> RDFNNLTKGLCTINSWHIYGKDNAVRIGED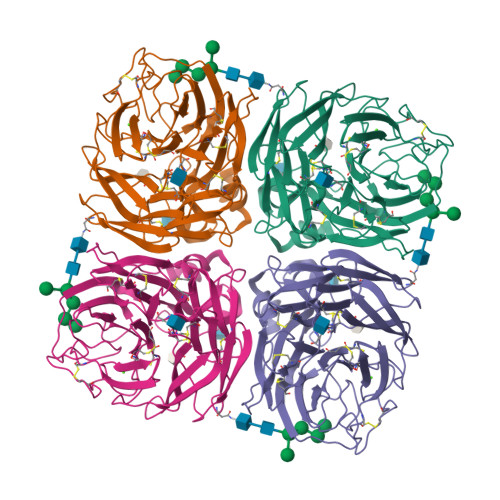SDVLVTREPYVSCDPDECRFYALSQGTTIRGKHSNGTIHDRSQYRALISWPLSSPPTVYNSRVECIGWSSTSCHDGKTRMSICISGPNNNASAVIWYNRRPVTEINTWARNILRTQESECVCHNGVCPVVFTDGSATGPAETRIYYFKEGKILKWEPLAGTAKHIEECSCYGERAEITCTCRDNWQGSNRPVIRIDPVAMTHTSQYICSPVLTDNPRPNDPTVGKCNDPYPGNNNNGVKGFSYLDGVNTWLGRTISIALRSGYEMLKVPNALTDDKSKPTQGQTIVLNTDWSGYSGSFMDYWAEGECYRACFYVELIRGRPKEDKVWWTSNSIVSMCSSTEFLGQWDWPDGAKIEYFL>[4x]TKHKERVMYYGKGDVFAYRTYLKPLT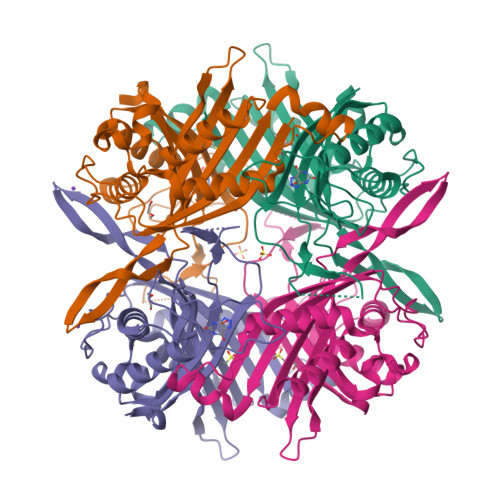GVRTIPESPFSGRDHILFGVNVKISVGGTKLLTSFTKGDNSLVVATDSMKNFIQKHLASYTGTTIEGFLEYVATSFLKKYSHIEKISLIGEEIPFETTFAVKNGNRAASELVFKKSRNEYATAYLNMVRNEDNTLNITEQQSGLAGLQLIKVSGNSFVGFIRDEYTTLPEDSNRPLFVYLNIKWKYKNTEDSFGTNPENYVAAEQIRDIATSVFHETETLSIQHLIYLIGRRILERFPQLQEVYFESQNHTWDKIVEEIGESEGKVYTEPRPPYGFQCFTVTQEDLPHENILMFSDE>[6x]MAMWTPQTGKLYLPPTTPVAKVQSTDEYVYPTSLFCHAHTDRLLTVGHPFFSVIDNDKVTVPKVSGNQYRVFRLKFPDPNKFALPQKDFYDPEKERLVWRLRGLEIGRGGPLGIGTTGHPLFNKLGDTENPNKYQQGSKDNRQNTSMDP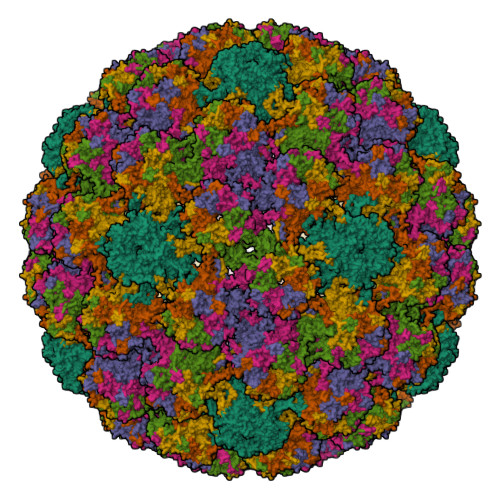KQTQLFIVGCEPPTGEHWDVAKPCGALEKGDCPPIQLVNSVIEDGDMCDIGFGNMNFKELQQDRSGVPLDIVSTRCKWPDFLKMTNEAYGDKMFFFGRREQVYARHFFTRNGSVGEPIPNSVSPSDFYYAPDSTQDQKTLAPSVYFGTPSGSLVSSDGQLFNRPFWLQRAQGNNNGVCWHNELFVTVVDNTRNTNFTISQQTNTPNPDTYDSTNFKNYLRHVEQFELSLIAQLCKVPLDPGVLAHINTMNPTILENWNLGFVPPPQQSISDDYRYITSSATRCPDQNPPKEREDPYKGLIFWEVDLTERFSQDLDQFALGRKFLYQAGIRTAVTGRGVKRAASTTSASSRRVVKRKRGSK>MEPDLFYILGNKVRRDLLSHLTCMECYFSLLSSKVSVSSTAVAKHLKIMEREGVLQSYEKEERFIGPTKKYYKISIAKSYVFTLTPEMFWYKGLDLGDAELRDFEISLSGLDTEPSTLKEMITDFIKANKELEKVLEAFKTIESYRSSL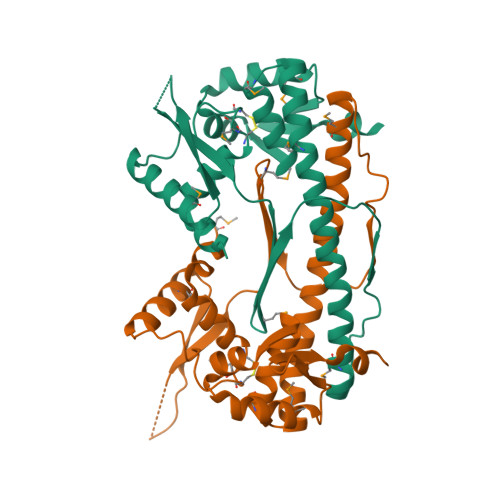MRKIKEAYLKEIGDMTQLAILHYLLLNGRATVEELSDRLNLKEREVREKISEMARFVPVKIINDNTVVLDEDQILRGEGNEED[4x]PROPYL ACETATE | C5 H10 O2 | 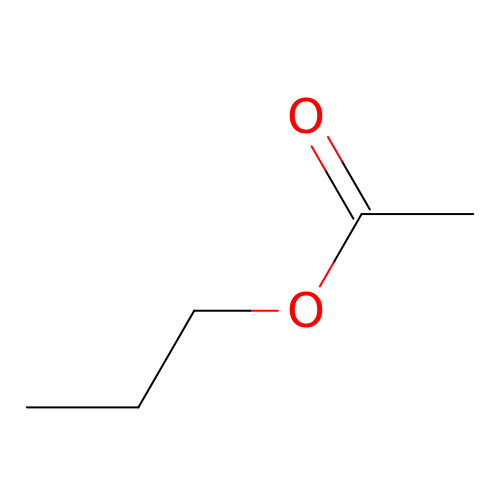YKYONYBAUNKHLG-UHFFFAOYSA-N>[4x]MGHHHHHHMVLADLGRKITSALRSLSNATIINEEVLNAMLKEVCTALLEADVNIKLVKQLRENVKSAIDLEEMASGLNKRKMIQHAVFKELVKLVDPGVKAWTPTKGKQNVIMFVGLQGSGKTTTCSKLAYYYQRKGWKTCLICADTFRAGAFDQLKQNATKARIPFYGSY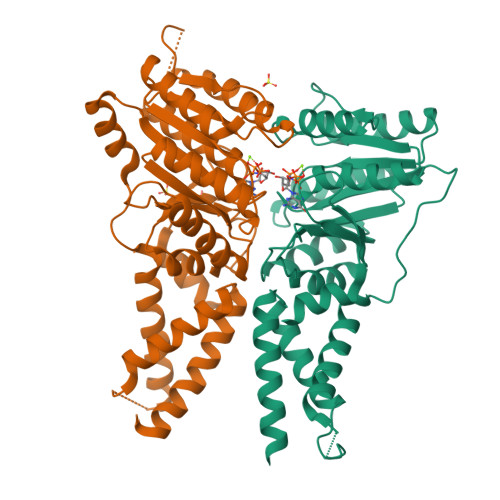TEMDPVIIASEGVEKFKNENFEIIIVDTSGRHKQEDSLFEEMLQVANAIQPDNIVYVMDASIGQACEAQAKAFKDKVDVASVIVTKLDGHAKGGGALSAVAATKSPIIFIGTGEHIDDFEPFKTQPFISKLLG;>MGSLSREDMESVLDKMRDHLIAKNVAADIAVQLCESVANKLEGKVMGTFSTVTSTVKQALQESLVQILQPQRRVDMLRDIMDAQRRQRPYVVTFCGVNGVGKSTNLAKISFWLLENGFSVLIAACDTFRAGAVEQLRTHTRRLSALHPPEKHGGRTMVQLFEKGYGKDAAGIAMEAIAFARNQGFDVVLVDTAGRMQDNAPLMTALAKLITVNTPDLVLFVGEALVGNEAVDQLVKFNRALADHSMAQTPRLIDGIVLTKFDTIDDKVGAAISMTYITSKPIVFVGTGQTYCDLRSLNAKAVVAALMKAHHHHHH[4x]> GAGCAGACGTGACAGCACTCA;> TGTCA;> TCTGAGTGC;> CGTCTGC

In this work, we exhaustively probe the ability of all 36 immobile HJ sequences to form DNA crystals in two different designed systems. Three separate self-assembling DNA crystal systems are described in this report: the “4 × 5” and “4 × 6” designs (collectively referred to as the 4 × N systems), and a third construct with a “scrambled” sequence variant of the 4 × 6 lattices. Self-assembly was mediated by three constituent oligonucleotides: (S1) containing four sequence repeats of either 5 or 6 bases; (S2) composed of 21 bases containing complementary regions to both (S1); and (S3) which forms the second junction crossover. The HJ serves as the fundamental component at the core of each unit, and the ultimate assembly of the full lattice is facilitated by the complementary 2-base sticky ends that tail each duplex.

Each asymmetric unit could be defined as either a HJ containing 10 and 11 bp on each arm, or as a 21-bp linear duplex. The 4 × 5 system robustly crystallized with 75% of the junctions, and we obtained crystals in all but 9 of 36 sequences. Of the resulting structures, 18 exhibited P32 symmetry with average cell dimensions a = b = 68.85 Å c = 60.09 Å, with only nine retaining the original P3221 symmetry with average cell edges a = b = 68.17 Å c = 60.60 Å. Although the cell parameters between the two symmetries were virtually indistinguishable, the differences between the periodicity of the lattices is dramatic, with vastly different cavity sizes.> GYQDPARSVRHIAIPAHRGLITDRNGEPLAVSTPVTTLWANPKELMTAKERWPQLAAALGQDTKLFADRIEQNAEREFIYLVRGLTPEQGEGVIALKVPGVYSIEEFRRFYPAGEVVAHAVGFTDVDDRGREGIELAFDEWLAGVPGKRQVLKDRRGRVIKDVQVTKNAKPG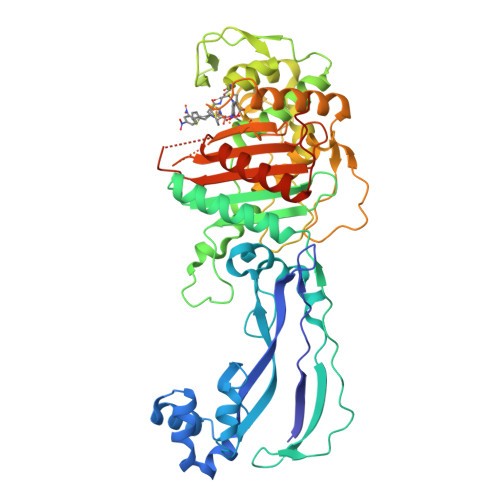KTLALSIDLRLQYLAHRELRNALLENGAKAGSLVIMDVKTGEILAMTNQPTYNPNNRRNLQPAAMRNRAMIDVFEPGSTVKPFSMSAALASGRWKPSDIVDVYPGTLQIGRYTIRDVSRNSRQLDLTGILIKSSNVGISKIAFDIGAESIYSVMQQVGLGQDTGLGFPGERVGNLPNHRKWPKAETATLAYGAGLSVTAIQLAHAYAALANDGKSVPLSMTRVDRVPDGVQVISPEVASTVQGMLQQVVEAQGGVFRAQVPGYHAAGKSGTARKVSVGTKGYRENAYRSLFAGFAPATDPRIAMVVVIDEPSKAGYFGGLVSAPVFSKVMAGALRLMNVPPDNLPTATEQQQVNAAPAKGGRG>[2x]MSAPV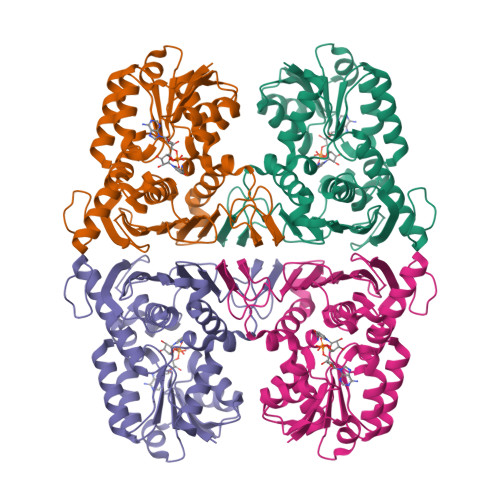RVGVVGAGFMGGVHAEVVAAHPGARLEAVHDLDPAAARDLAERFRAERAEPSWADLLADPAIDLLIITTPNGLHHRQAAEALRAGKHVLVEKPLGVTPEQVAELVELAGRHDRVLAHGSNFVHSPKFVRARQLVADTEAFGRPHLVRVVFRNSGPEAAWAASKDLAGGGALLDLGCHAVELCRWLLDGADVESVSARLQRVRPPHDAEADRASGTAGTARVALEDQALLVMEFADGAVGQCDVSWVTQGGEQVTAEIIGTKGRVEVDLWTGMGLRAYSDKGYQDVWDPEQGWVHPEWEWIRASGYYHQDGTVIEAVGQGIPLTHGPAEALASARVLATGYRSHAEGRVLRLSGAPVGPGASTTAAGSEKLAAALEHHHHHH>[6x]MAHHHHHHMKISDGNWLIQPGLNLIQPVQVYEVEQQGNEMVVYAAPRDVRERAWQLDTPLFTLRFFSPQEGIIGVRMEHFQGALDNSPHYPLNVQKDVHVEIENTAEFAELKSGSLSVRVTKGEFWALDFLRDGVRITGSQLKNNGYVQDSKTQRNYMFERLDLGVGETVYGLGERFTALVRNGQTVETWNEDGGTSTEQSYKNIPFYLTNRGYGVLVNHPQRVSFEVGSEKVSKVQFSVEGEYLEYFVIDGPTPKAVLNRYTQFTGRPALPPAWSFGLWLTTSFTTNYDEATVNSFIDGMAERHLPLHVFHFDCFWMKAFQWCDFEWDPLTFPDPEGMIKRLKAKGLKVCVWINPYIGQRSPVFKELKEKGYLLKRPDGSLWQWDKWQPGLAIYDFTNPEACQWYASKLKGLVAMGVDCFKTDFGERIPTDVQWFDGSDPQKMHNHYAFIYNELVWKVLKETVGEQEAVLF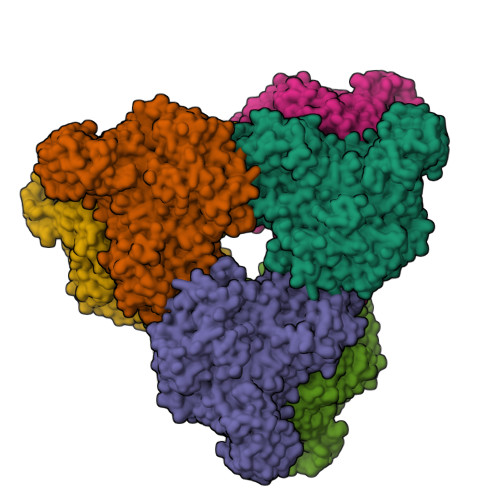ARSASVGAQQFPVHWGGDCYANYESMAESLRGGLSIGMSGFGFWSHDIGGFENTAPAHVYKRWCAFGLLSSHSRLHGSKSYRVPWAYDEESCDVVRHFTQLKCRMMPYLYRQAALANEFGTPMLRAMMLEFPDDPACDYLDRQYMLGDSVLVAPVFSEAGEVQFYLPEGRWTHLWHNDELPGSRWHKQRHDALSLPVYVRDNTLLALGNNDQKPDYAWHEGTAFQLFQLGDGNETVCQVPAADGSAIFTLKAKRQGNTITVSGEGEARGWTLCLRNIPQIAGVEGGTQAGSELGVVVSAQGNALTISL3-(2-methoxyphenyl)benzoic acid | C14 H12 O3 | 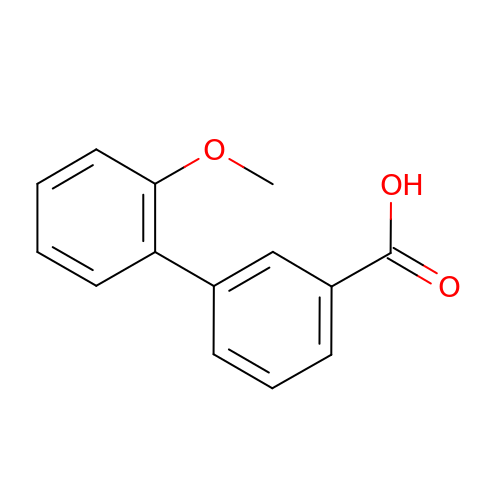COUUHAJQLHMNJM-UHFFFAOYSA-N> SIMIPTHSTGGLHQGTEGWHRTNNVKNFLMRVEKWSLRNPGYTALIAILGWTLGTTTAQKVI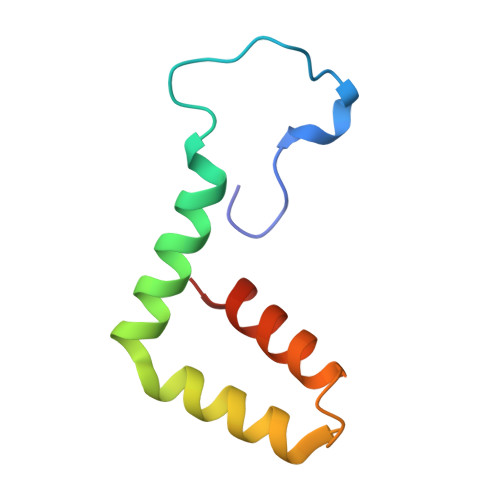FIALLLMIAPVYG> MALKKNTHNKSTKRVTKHPSLKTLTHKQIHTTIFVKSTTPYVSALKRINKFLDSVHKQGSSYVAVLGMGKAVEKTLALGCHFQDQKNKKIEVY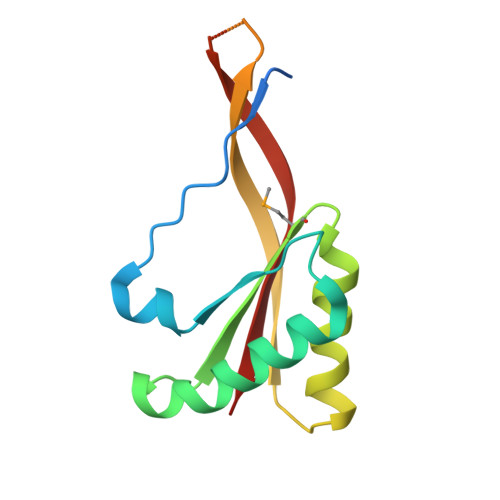TKTIEVLDEVITEGQADIDMESDVEDDDKETQLKKRAVSGVELRIYV(3R)-3-biphenyl-4-yl-1-azabicyclo[2.2.2]octan-3-ol | C19 H21 N O | 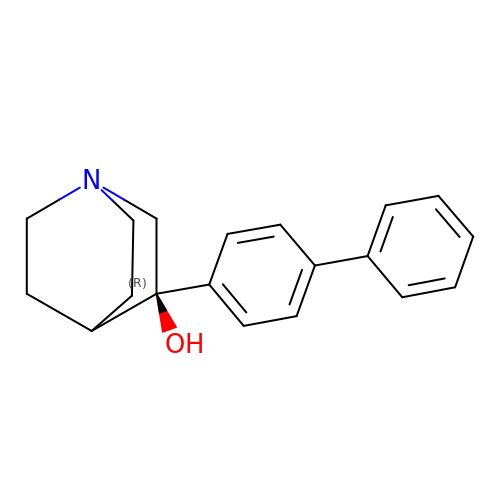WPCQYFUQHBLGAX-IBGZPJMESA-N>[2x]GMDVFSEYLAGIADPFHRERTEEVLTWIKNKYPNLHTEIKWNQPMFTDHGTFIIGFSVSK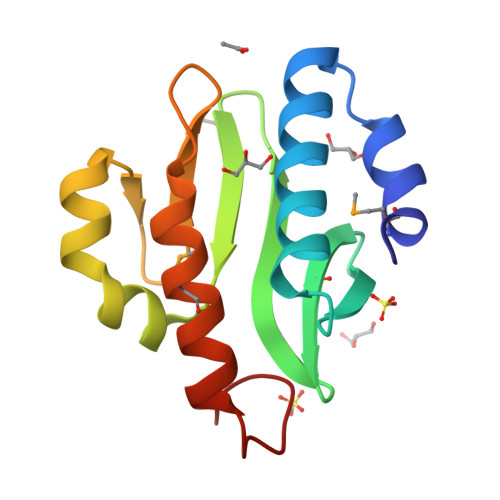KHLAVAPEKVTIAHVEDDIVKAGYDYTEQLIRIPWNGPVDYTLLEKMIEFNILDKADCSTFWRK>[3x]GSHMSNTQTVLPWTGLNTPSGVAVDSAGTVYVTDHGNNRVVKLAAGSNTQTVLPFTGLNTPSGVAVDSAGTVYVTDHGNNRVVKLAAGSNTQTVLPWTGLNTPSGVAVDSAGTVYVTDHGNNRVVKLAAGSNTQTVLPFTGLNTPSGVAVDSAGTVYVTDHGNNR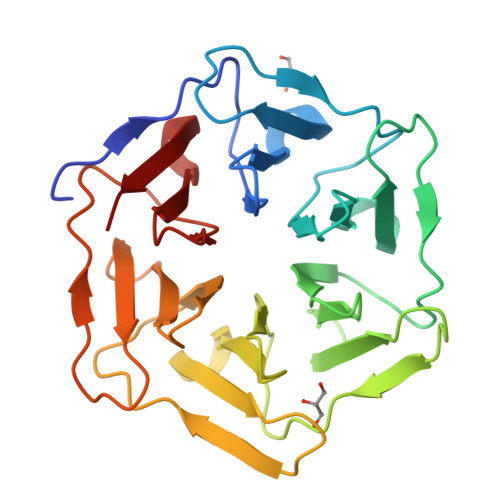VVKLAAGSNTQTVLPWTGLNTPSGVAVDSAGTVYVTDHGNNRVVKLAAGSNTQTVLPFTGLNTPSGVAVDSAGTVYVTDHGNNRVVKLAAG>[2x]RELGSNMVHPNVICDGCNGPVVGTRYKCSVCPDYDLCSVCEGKGLHRGHTKLAFPSP

Sequestosome 1 (SQSTM1 or p62) mediates cell proliferation, survival, and death through multiple signaling programs, including autophagy and metabolism. Structurally, p62 contains six functional motifs: an N-terminal PKC-binding PB1 (Phox and Bem1p) domain, the central ZZ and TB modules, a LC3-interacting region (LIR), a Keap1-binding region (KIR), and the C-terminal ubiquitin associated (UBA) domain. Following binding to the ubiquitinated cargos, p62 undergoes oligomerization and delivers the cargo aggregates to the autophagosome via interacting with the autophagosomal membrane protein LC3. Here, we report the structural basis underlying specific recognition of Nt-R substrates by the ZZ domain of p62.

To gain insight into the molecular mechanism by which p62 recognizes Nt-R substrates, we determined the atomic-resolution structure of the p62ZZ-RE complex. We designed and crystallized a chimeric construct containing the Arg-Glu sequence fused via a short linker to the N-terminus of the ZZ domain of p62 (aa 120–171) (hereafter referred to as RE-ZZ). In the structure, two RE-ZZ molecules form a complex in which the RE residues of one molecule are bound by the ZZ domain of another molecule, whereas the linker residues are flexible and have no contact with either ZZ domain. An extensive network of salt bridges and hydrogen bonds stabilizes the p62ZZ-RE complex. The Nt-R is bound in a highly negatively charged groove lined with the residues D129, N132, D147, and D149 of p62. The guanidinium moiety of Arg1 is constrained by a salt bridge with the carboxyl group of D129 and hydrogen bonds with the oxygen atom of the carboxamide group of N132. Notably, the α-amino-terminal NH3+ group of Arg1 is bound via a set of intermolecular contacts, including salt bridges and hydrogen bonds with the carboxyl groups of D129 and D149 and the backbone carbonyl group of I127. In addition, the carbonyl group of Arg1 is hydrogen bonded to the backbone amide of I127. The complex is further stabilized through the interactions involving degron’s Glu2. The side chain carboxyl group of Glu2 forms a salt bridge with the guanidinium moiety of R139, which in turn is restrained through electrostatic and hydrogen bonding contacts with D149, whereas the backbone amide of Glu2 donates a hydrogen bond to the carboxyl group of D147.>MGQYKKLWYLLFAVLAVCFTILGYMGSEVYKKAPPYPEQVVSASGKVLMAKDDILAGQSAWQTTGGMEVGSVLGHGAYQAPDWTADWLHRELSAWLDLT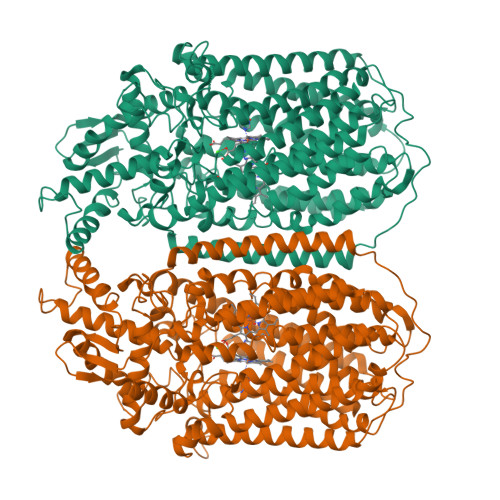AQQTYGKKFDEVSPEEQAVLKTRLADEYRNQSRIKEDGSVVISDTRVKAIESILPYYHGVYGDDPALQTTREHFAMKNNTLPSQEAREKLFDFFFWTSWSASTNRPDETFTYTNNWPHEPLINNVPTTENYMWSFTSVVLLLMGIGLLMWGYSFLTKHEEVEVPTEDPISKVQLTPSQKALGKYVFLTVALFVVQVLLGGLTAHYTVEGQGFYGIDEALGFEMSDWFPYALTRTWHIQSAIFWIATGFLTAGLFLAPIVNGGKDPKFQRAGVNFLYIALFIVVGGSYAGNFFALTHILPPEFNFWFGHQGYEYLDLGRFWQLLLMVGLLLWLFLMLRCTVSAFKEKGVDKNLLAIFVASMVGVGVFYAPGLFYGEKSPIAVMEYWRWWVVHLWVEGFFEVFATAAFAFVFYNMGFVRRSTATASTLAAAAIFMLGGVPGTLHHLYFSGSTSASMAIGACFSALEVVPLVLLGREAYEHWSYQHLSEWAKRLRWPLMCFVAVAFWNMIGAGVFGFLINPPISLFYIQGLNTSAVHAHAALFGVYGFLALGFVLLVARYLKPNVQFDDKLMTWGFWLLNGGLVGMIAISLLPVGVIQAYASITHGLWYARSEEFLQMEILDTLRWVRTAADLIFIGGAICVAIQATKIVFGRDK[2x]The most prominent such domain has been identified by bioinformatics as part of non-structural protein 3 (Nsp3) of the virus and appropriately named the “SARS-unique domain” (SUD). SUDcore turns out to consist of two subdomains, SUD-N (Nsp3 residues 389–517) and SUD-M (525–652), each exhibiting the fold of a macrodomain. The two subdomains are connected by a flexible linker (residues 518–524) and a disulfide bond. Instead, we have demonstrated that full-length SUD and SUDcore bind oligodeoxynucleotides and oligoribonucleotides that form G-quadruplexes.

In this communication, we describe the crystal structures at 2.2 Å and 2.8 Å resolution (monoclinic and triclinic form, respectively) of the core of the SARS-unique domain (SUDcore, Nsp3 residues 389–652). Two crystal forms were observed under identical crystallization conditions: Form-1 crystals were monoclinic (space group P21, two SUDcore molecules per asymmetric unit) and diffracted X-rays to 2.2 Å resolution; form-2 crystals were triclinic (space group P1, four SUDcore molecules per asymmetric unit) and diffracted to 2.8 Å. Both structures were determined by molecular replacement. The r.m.s. deviations (on Cα atoms) between the models derived from the two different crystal structures are around 0.7 Å. In both crystal forms, SUDcore displays the same head-to-tail dimer, with the SUD-N subdomain of monomer A interacting with the SUD-M subdomain of monomer B, and vice versa. Approximately 1130 Å2 of solvent-accessible surface per monomer is buried upon dimerization. Involving ∼10 hydrogen bonds and four well-defined salt-bridges (AspB440…ArgA554, ArgB473…GluA619, ArgB554…AspA440, and GluB619…ArgA473), interactions between the monomers are largely hydrophilic. As to be expected, the structures of the monomers are very similar to one another, with r.m.s.d. values (for Cα atoms) of 0.58 Å between monomers A and B of the monoclinic crystal form, and 0.11–0.37 Å between monomers A–D of the triclinic form. In all six independent copies of the SUDcore monomer, residue Val611 adopts forbidden conformational angles. The side chain makes a hydrophobic contact across the subdomain interface and is also contacting the side chain of Phe406 of a symmetry-related SUDcore dimer in the crystal lattice in the monoclinic crystal form (this also applies to two of the four monomers in the triclinic form).

>[2x]KIKACIDEVTTTLEETKFLTNKLLLFADINGKLYHDSQNMLRGEDMSFLEKDAPYMVGDVITSGDITCVVIPSKKAGGTTEMLSRALKKVPVDEYITTYPGQGCAGYTLEEAKTALKKCKSAFYVLPSEAPNAKEEILGTVSWNLREMLAHAEETRKLMPICMDVRAIMATIQRKYKGIKIQEGIVDYGVRFFFYTSKEPVASIITKLNSLNEPLVTMPIGYVTHGFNLEEAARCMRSLRAPAVVSVSSPDAVTTYNGYLTSSS>MWKDKEFQVLFVLTILTLISGTIFYSTVEGLRPIDALYFSVVTLTTVGCDISPQTDFGKIFTILYIFIGIGLVFGFIHKLAVNVQLPSILSNLVPR[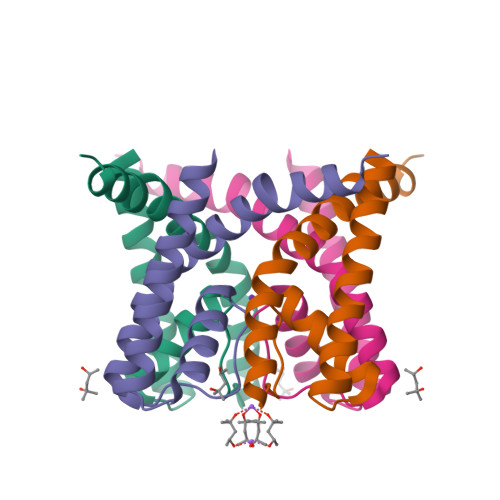2x]> SAPAAATPSLKVLTYNTFLMSTGLYPNWGQEHRAREIAAAGFFQGNDVVVLQEAFDNAAADGLKAAAADRYPYQTPVVGRSRDGWDATGGKYSATTPEDGGVTVLSKWPIVRK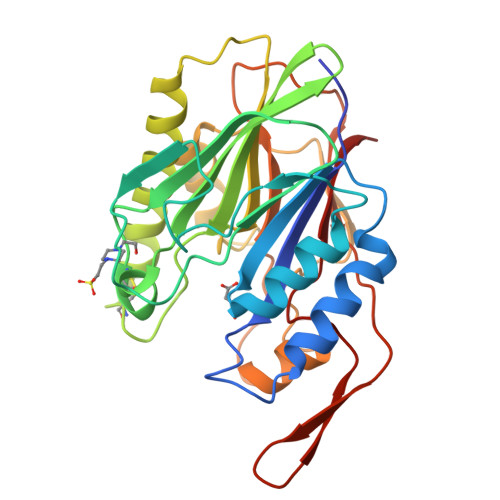EQVIFNDACGADWWSNKGFAYVVLNVGGTRVHVVGTHAQSTDSGCAAGEAAADRSRQFRQIDAFLDAKNIPADEQVMLAGDLNVDSHSAEYASMLADGDLAPADSRAGHPYSFDTKENSIAAYRYPTDPREDLDYVLHRNGHARPAGWRNTVVQETSAPWTVSSWGKRYTYTDLSGHYPVIAGAN>MKGTCHCGAVEIEVELLNGFADARRCDCSFCRRRGAIAATARLSDLRVVRGAENLTLYQFGTRTAKHWFCRTCGIYTHHQRRSNPEEYGVNV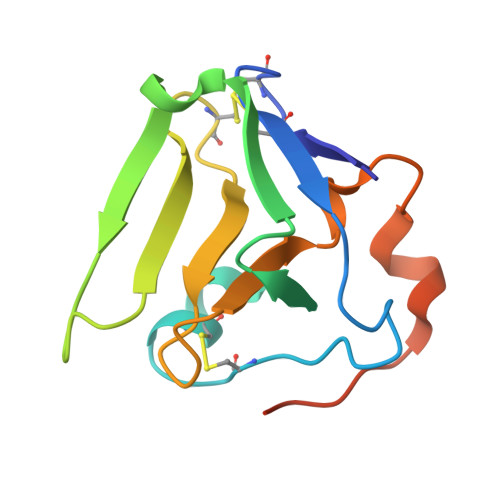AILEGVNPRDLGEVPWTDGVNHPSDR[8x]>MSQLALQMSSLGVEGEGIWLALGTIGMLLGMLYFIADGLDVQDPRQKEFYVITILIPAIAAASYLSMFFGFGLTEVSLANGRVVDVYWARYANWLFTTPLLLLDIGLLAGASQRDIGALVGIDAFMIVTGLVATLTKVVVARYAFWTISTISMVFLLYYLVAVFGEAVSDADEDTRSTFNALRNIILVTWAIYPVAWLVGTEGLALTGLYGETLLFMVLDLVAKVGFGFILLRSRAIMGGGSEPTPSAQETAADLEH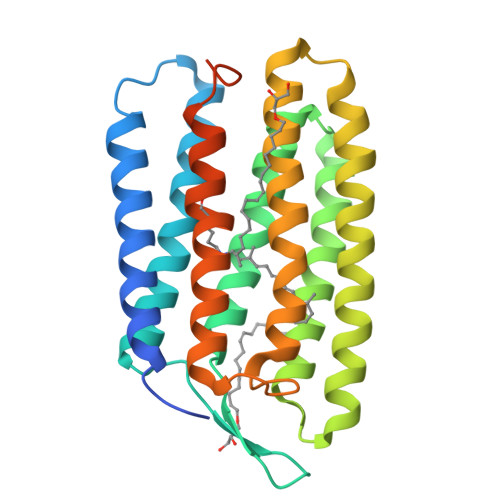HHHHH[2x]>[15x]MSMYTTAQLLAANEQKFKFDPLFLRLFFRESYPFTTEKVYLSQIPGLVNMALYVSPIVSGEVIRSRGGSTSEFTPGYVKPKHEVNPQMTLRRLPDEDPQNLADPAYRRRRIIMQNMRDEELAIAQVEEMQAVSAVLKGKYTMTGEAFDPVEVDMGRSEENNITQSGGTEWSKRDKSTYDPTDDIEAYALNASGVVNIIVFDPKGWALFRSFKAVKEKLDTRRGSNSELETAVKDLGKAVSYKGMYGDVAIVVYSGQYVENGVKKNFLPDNTMVLGNTQARGLRTYGCIQDADAQREGINASARYPKNWVTTGDPAREFTMIQSAPLMLLADPDEFVSVQLA;>[12x]MKTPTIPTLLGPDGMTSLREYAGYHGGGSGFGGQLRSWNPPSESVDAALLPNFTRGNARADDLVRNNGYAANAIQLHQDHIVGSFFRLSHRPSWRYLGIGEEEARAFSREVEAAWKEFAEDDCCCIDVERKRTFTMMIREGVAMHAFNGELFVQATWDTSSSRLFRTQFRMVSPKRISNPNNTGDSRNCRAGVQINDSGAALGYYVSEDGYPGWMPQKWTWIPRELPGGRASFIHVFEPVEDGQTRGANVFYSVMEQMKMLDTLQNTQLQSAIVKAMYAATIESELDTQSAMDFILGANSQEQRERLTGWIGEIAAYYAAAPVRLGGAKVPHLMPGDSLNLQTAQDTDNGYSVFEQSLLRYIAAGLGVSYEQLSRNYAQMSYSTARASANESWAYFMGRRKFVASRQASQMFLCWLEEAIVRRVVTLPSKARFSFQEARSAWGNCDWIGSGRMAIDGLKEVQEAVMLIEAGLSTYE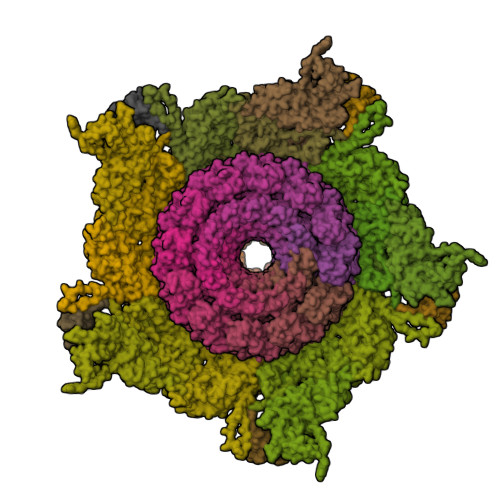KECAKRGDDYQEIFAQQVRETMERRAAGLKPPAWAAAAFESGLRQSTEEEKSDSRAA;>MTSKETFTHYQPQGNSDPAHTATAPGGLSAKAPAMTPLMLDTSSRKLVAWDGTTDGAAVGILAVAADQTSTTLTFYKSGTFRYEDVLWPEAASDETKKRTAFAGTAISIV[20x];>[6x]MKHTELRAAVLDALEKHDTGATFFDGRPAVFDEADFPAVAVYLTGAEYTGEELDSDTWQAELHIEVFLPAQVPDSELDAWMESRIYPVMSDIPALSDLITSMVASGYDYRRDDDAGLWSSADLTYVITYEM;>MTRQEELAAARAALHDLMTGKRVATVQKDGRRVEFTATSVSDLKKYIAELEVQTGMTQRRRGPAGFYV[12x];>MADFDNLFDAAIARADETIRGYMGTSATITSGEQSGAVIRGVFDDPENISYAGQGVRVEGSSPSLFVRTDEVRQLRRGDTLTIGEENFWVDRVSPDDGGSCHLWLGRGVPPAVNRRR[6x]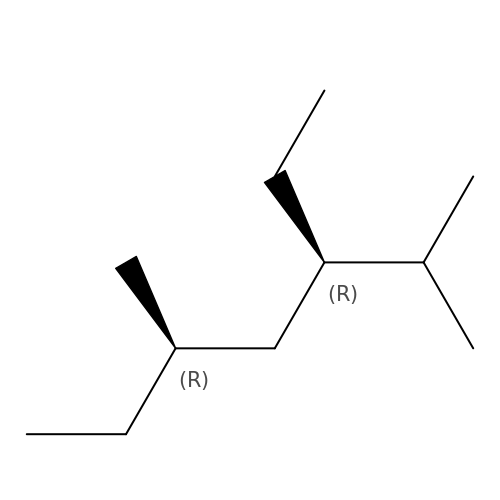(3R,5R)-3-ethyl-2,5-dimethylheptane | C11 H24 | DEZOXTLNRYCKNK-GHMZBOCLSA-N> VRLPGLAAMRQGTRLFTPEQGEDLRE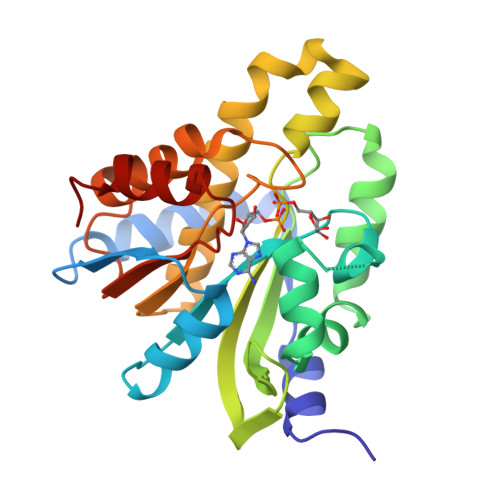ALRRRRGSFQTTCEVTSETTFAAARRLREKASALAALNFASAKNPGGGFLGGAQAQEEDLCRGSGLYFSLTSPQAEPYYAVNRQSHSALYTDHLIYSPQVPIFRDDAGQLLPAPVPVNIITAPAPNAGAVAQSRPEQLPQVLPTLRERARRVLGVAAWMEQTHLVLGAWGCGVFRNDPAGVARTFRELLEGEAQGAFEHVTFAVLDNHPQHPKLGAFRRELESLC> S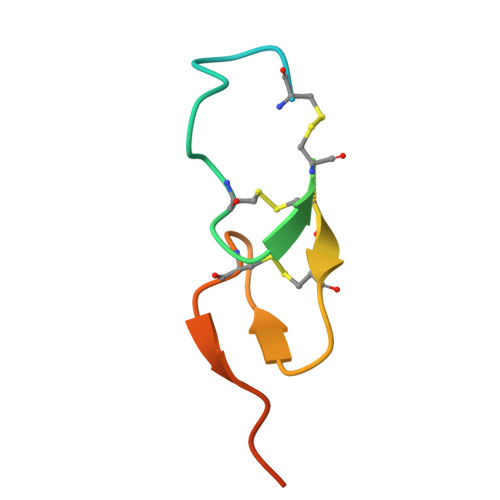EGPIALKFSHLCLEDHNSYCINGACAFHHELEKAICRCFTGYTGERCEHLTLTSYAVDSY>[2x]GSPGILMASQGTKRSYEQMETGGERQNATEIRASVGRMVGGIGRFYIQMCTELKLSDQEGRLIQNSITIERMVLSAFDERRNRY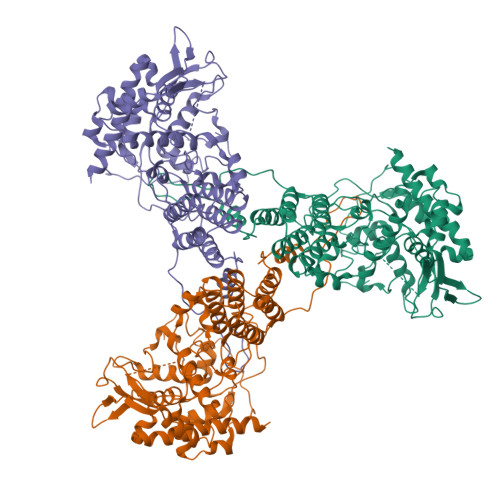LEEHPSAGKDPKKTGGPIYRRRDGKWVRELILYDKEEIRRIWRQANNGEDATAGLTHMMIWHSNLNDATYQRTRALVRTGMDPRMCSLMQGSTLPRRSGAAGAAIKGVGTMVMELIRMIKRGINDRNFWRGENGRRTRIAYERMCNILKGKFQTAAQKAMMDQVRESRNPGNAEIEDLIFLARSALILRGSIAHKSCLPACVYGLAVASGYDFEREGYSLVGIDPFRLLQNSQVFSLIRPNENPAHKSQLVWMACHSAAFEDLRVSSFIRGTRVIPRGQLSTRGVQIASNENVEAMDSSTLELRSRYWAIRTRSGGNTNQQRASAGQISVQPTFSVQRNLPFERATIMAAFKGNTEGRTSDMRTEIIRMMESARPEDVSFQGRGVFELSDEKATNPIVPSFDMSNEGSYFFGDNAEEYDN>[6x]SSSESLSIIDVASDQNLFQTFIKEWRCKKRFSISLACEKIRSLTSSKTATIGSRFKQASSPQEIPIRDDGFPIKGCDDTLVVGLAVCWGGRDAYYFSLQKE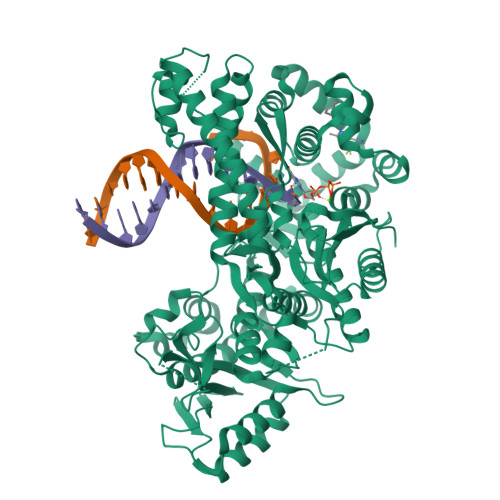QKHSEISASLVPPSLDPSLTLKDRMWYLQSCLRKESDKECSVVIYDFIQSYKILLLSCGISLEQSYEDPKVACWLLDPDSQEPTLHSIVTSFLPHELPLLEGMETSQGIQSLGLNAGSEHSGRYRASVESILIFNSMNQLNSLLQKENLQDVFRKVEMPSQYCLALLELNGIGFSTAECESQKHIMQAKLDAIETQAYQLAGHSFSFTSSDDIAEVLFLELKLPPNREMKNQGSKKTLGSTRRGIDNGRKLRLGRQFSTSKDVLNKLKALHPLPGLILEWRRITNAITKVVFPLQREKCLNPFLGMERIYPVSQSHTATGRITFTEPNIQNVPRDFEIKMGGMPFSISMRHAFVPFPGGSILAADYSQLELRILAHLSHDRRLIQVLNTGADVFRSIAAEWKMIEPESVGDDLRQQAKQICYGIIYGMGAKSLGEQMGIKENDAACYIDSFKSRYTGINQFMTETVKNCKRDGFVQTILGRRRYLPGIKDNNPYRKAHAERQAINTIVQGSAADIVKIATVNIQKQLETFHSTFKSHGHREGMLQSDQTGLSRKRKLQGMFCPIRGGFFILQLHDELLYEVAEEDVVQVAQIVKNEMESAVKLSVKLKVKVKIGASWGELKDFDV>SLLENAEEEKERQI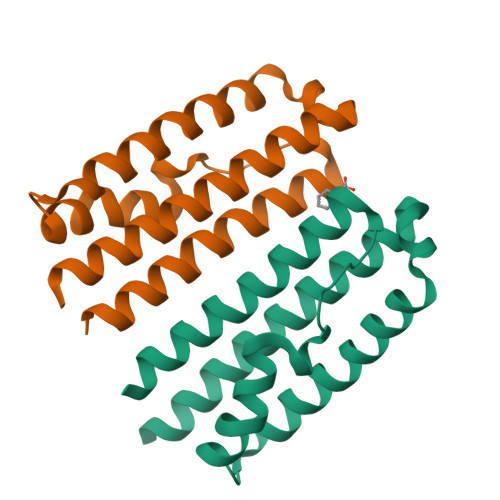ASILSWEIDIIYKILLDSDLGSSLPLSQADFGLWFNHKGRHYFSGIAEVGHISRLIQDFDGIFNQTMRNTRNLNNRSLRVKFLLQIRNTVSQIITLLRELFEEVSRHEVGMD[2x]> SMQPPIAKPGETWILQAKRSDEFNVKDATKWNFQTENYGVWSWKNENATVS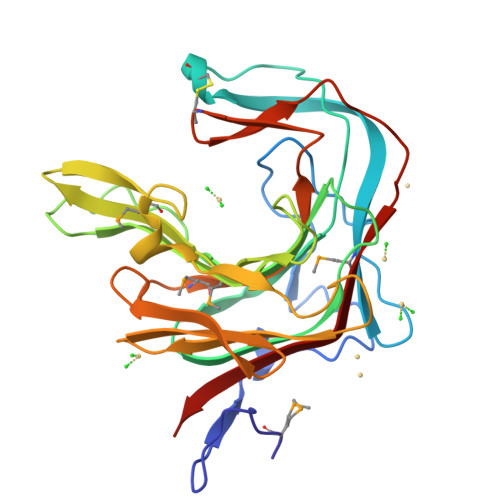KGKLKLTTKRESHQRTFWDGCNQQQVANYPLYYTSGVAKSRATGNYGYYEARIKGASTFPGVSPAFWMYSTIDRSLTKEGDVQYSEIDVVELTQKSAVRESDHDLHNIVVKNGKPTWMRPGSFPQTNHNGYHLPFDPRNDFHTYGVNVTKDKITWYVDGEIVGEKDNLYWHRQMNLTLSQGLRAPHTQWKCNQFYPSANKSAEGFPTSMEVDYVRTWVKV> GPLGSMKLLVVDDSSTMRRIIKNTLSRLGYEDVLEAEHGVEAWEKLDANADTKVLITDWNMPEMNGLDLVKKVRSDSRFKEIPIIMITTEG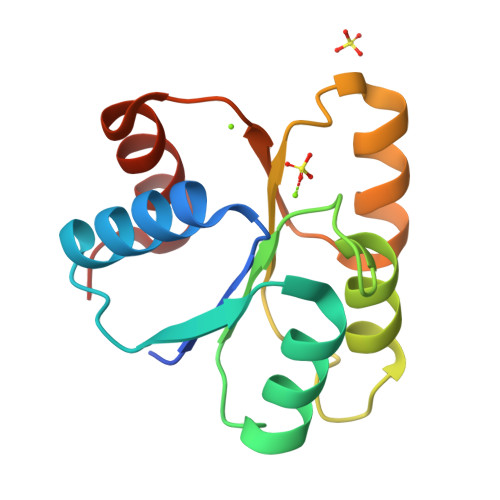GKAEVITALKAGVNNYIVKPFTPQVLKEKLEVVLGTND(2R)-2-(4-{[3-chloro-5-(trifluoromethyl)pyridin-2-yl]oxy}phenoxy)propanoic acid | C15 H11 Cl F3 N O4 | 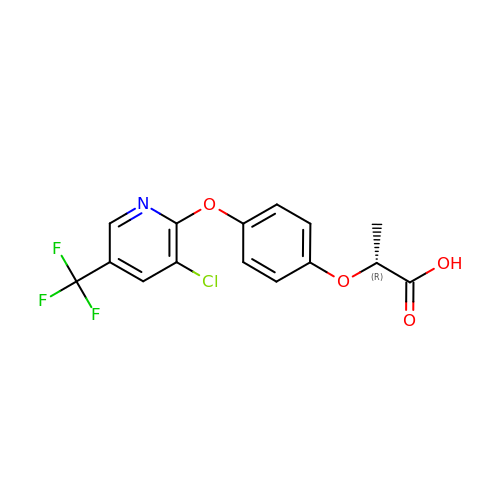GOCUAJYOYBLQRH-MRVPVSSYSA-N> MFEKQEVEQKKELKILEIIKEAIELGASDIHLTAGAPPAVRIDGYIKFLKDFPRLTPEDTQKLAYSVMSEKHRQKLEENGQVDFSFGVRGVGRFRANVFYQRGSVAAALRSLPAEIPEFKKLGLPDKVLELCHRKMGLILVTGPTGSGKSTTIASMIDYINQTKSYHIITIEDPIEYVFKHKKSIVNQREVGEDTKSFADALRAALREDPDVIFVGEMRDLETVETALRAAETGHLVFGTLHTNTAIDTIHRIVDIFPLNQQEQV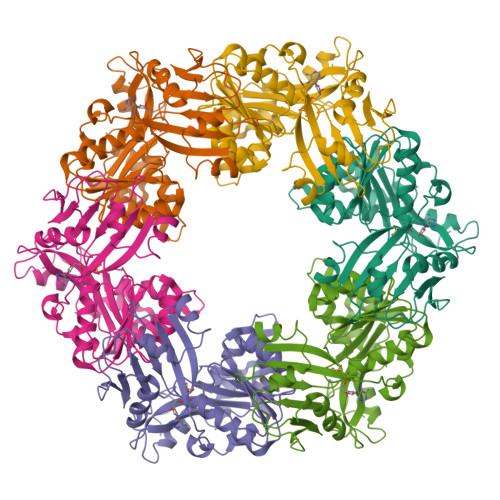RIVLSFILQGIISQRLLPKIGGGRVLAYELLIPNTAIRNLIRENKLQQVYSLMQSGQAETGMQTMNQTLYKLYKQGLITLEDAMEASPDPKELERMIRGGRHHHHHH> EDELYRQSLEIISRYLREQATGAKDTKPMGRSGATSRKALETLRRVGDGVQRNHETAFQGMLRKLDIKNEDDVKSLSRVMIHVFSDGVTNWGRIVTLISFGAFVAKHLKTI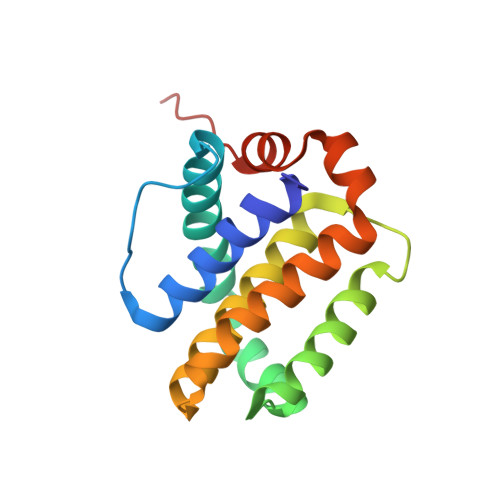NQESCIEPLAESITDVLVRTKRDWLVKQRGWDGFVEFFHVEDLEGG>MHHHHHHMLENKLGIINQLELNRVEERVSKENAKRLYDSGDIDRIEVGTFKGLSYIHNYLFEDIYEFAGKVRSQNISKGNFRFAPVMYLEIALEHIDKMPQRNLDEIVAKYVEMNIAHPFREGNGRATR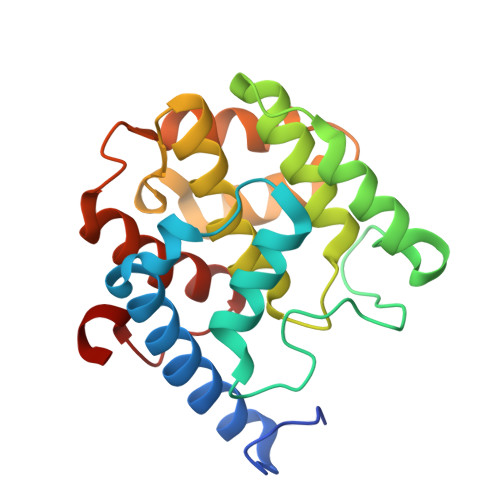IWLDLILKKELKRVVDWNLINKEDYLSAMERSPVKDLEIKYLISNALTDKINDREIFMKGIDISYYYEGYTEYNVDEL[4x]>[2x]MVRIYTLTLAPSLDSATITPQIYPEGKLRCTAPVFEPGGGGINVARAIAHLGGSATAIFPAGGATGEHLVSLLADENVPVATVEAKDWTRQNLHVHVEASGEQYRFVMPGAALNEDEFRQLEEQVLEIESGAILVISGSLPPGVK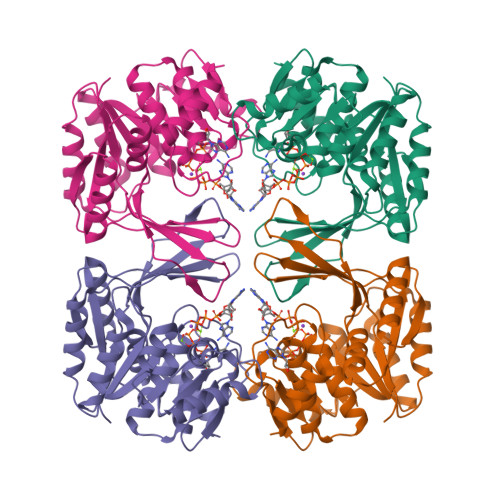LEKLTQLISAAQKQGIRCIVDSSGEALSAALAIGNIELVKPNQKELSALVNRELTQPDDVRKAAQEIVNSGKAKRVVVSLGPQGALGVDSENCIQVVPPPVKSQSTVGAGDSMVGAMTLKLAENASLEEMVRFGVAAGSAATLNQGTRLCSHDDTQKIYAYLSR> MTTLTRQDLNSAQVV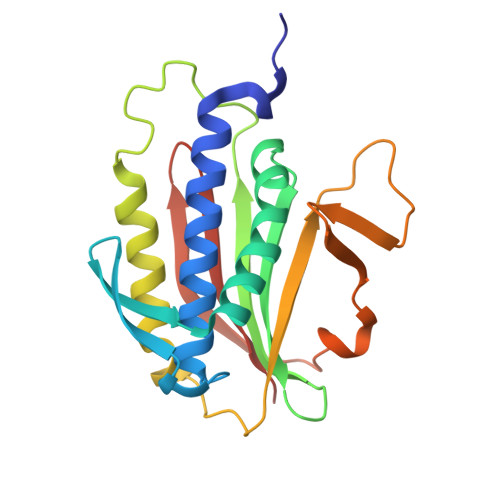ADVLSEFLEVAVHLILYVREVYPVGIFQKRKKYNVPVQMSCHPELNQYIQDTLHCVKPLLEKNDVEKVVVVILDKEHRPVEKFVFEITQPPLLSINSDSLLSHVEQLLRAFILKISKVDKVLDHNPPGCTFTVLVHTREAATRNMEKIQVIKDFPWILADEQDVHMHDPRLIPLKTMTSDILKMQLYVEERAHKNS>MAKVLQIGAGGVGGVVAHKMAMNREVFSHITLASRTLSKCQEIAQSIKAKGYGEIDITTVDADSIEELVALINEVKPQIVLNIALPYQDLTIMEACLRTGVPYLDTANYEHPDLAKFEYKEQWAFHDRYKEKGVMALLGSGFDPGVTNVFCAYAQKHYFDEIHEIDILDCNAGDHGYPFATNFNPEINLREVSSKGRYWENGEWIETEPMEIMQVWDYPEVGPKDSYLLYHEELESLVRNIKGLKRIRFFMTFGQSYLTHMRCLENVGMLRIDEIEVNGCKVVPIQVLKALLPDPASLASRTKGKTNIGCYIKGIKEGKARTIYIYNVCDHESCYREVNAQAISYTTGVPAMIGAKLMLEGKW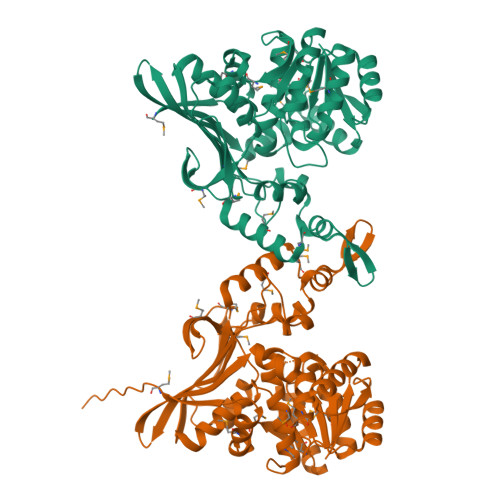SGKGVFNMEELDPDPFMDELNKQGLPWEVKEMEALEHHHHHH[2x]>MK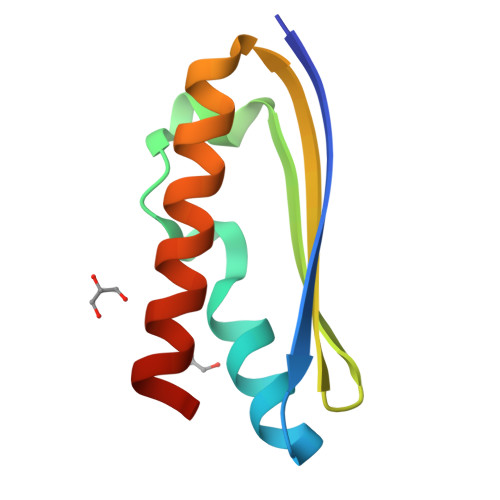IRAKVELTWEYEDEETAKAIANAVNVDNISIPEKLKKSLNLITFPDGARVVTKVKYEGEIESLVVALDDLIFAIKVAEEVLWSH[3x]>MAHHHHHHSSGLEVLFQGPMHVIKIGGSLTFNSKNLLSKLIELNKKIVLVPGGGNFADSVRELYDRTDLGELGAHKIATICTDITGIYFSEISGIKTANNLFDAKKILENENIVIILPSKIILSTDELPCSW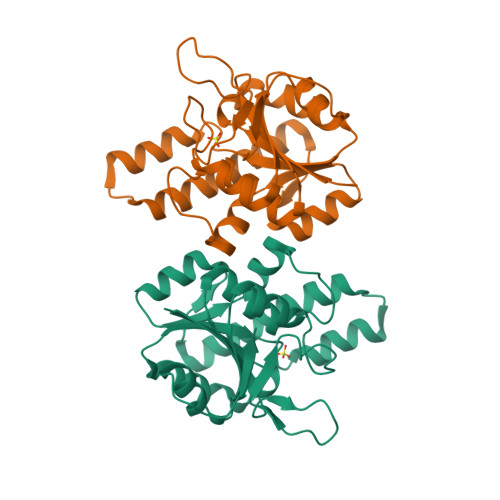SVTSDSFAAYIAKLLKSKVLIIATDVDGIYDKYPEGKLLNTINTKTIKGFTSVDKHLPKLISEYGIECFVVNGNHPERIKNILNDVSDTYTKITLE[2x]>MENFEIWVEKYRPRTLDEVVGQDEVIQRLKGYVERKNIPHLLFSGPPGTGKTATAIALARDLFGENWRDNFIEMNASDERGIDVVRHKIKEFARTAPIGGAPFKIIFLDEADALTADAQAALRRT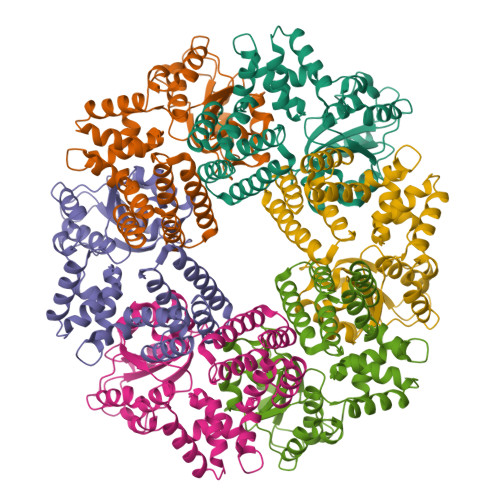MEMYSKSCRFILSCNYVSRIIEPIQSRCAVFRFKPVPKEAMKKRLLEICEKEGVKITEDGLEALIYISGGDFRKAINALQGAAAIGEVVDADTIYQITATARPEEMTELIQTALKGNFMEARELLDRLMVEYGMSGEDIVAQLFREIISMPIKDSLKVQLIDKLGEVDFRLTEGANERIQLDAYLAYLSTLAKK[6x]> SMDEAVGDLKQALPCVAESPTVHVEVHQRGSSTAKKEDINLSVRKLLNRHNIVFGDYTWTEFDEPFLTRNVQSVSIIDTELKVKDSQPIDLSACTVALHIFQLNEDGPSSENLEEETENIIAANHWVLPAAEFHGLWDSLVYDVEVKSHLLDYVMTTLLFSDKNVNSNLITWNRVVLLHGPPGTGKTSLCKALAQKLTIRLSSRYRYGQLIEINSH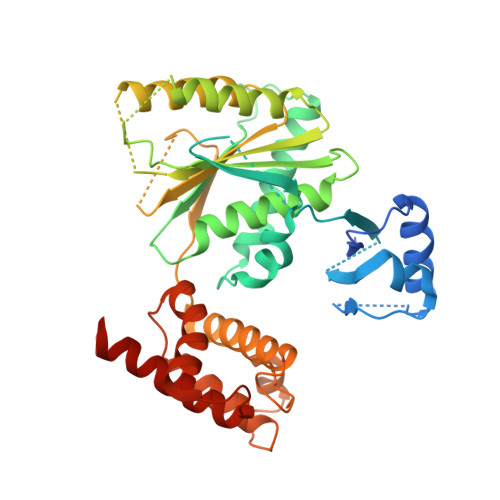SLFSKWFSESGKLVTKMFQKIQDLIDDKDALVFVLIDEVESLTAARNACRAGTEPSDAIRVVNAVLTQIDQIKRHSNVVILTTSNITEKIDVAFVDRADIKQYIGPPSAAAIFKIYLSCLEELMKCQIIYPRQQLLTLRELEMIGFIENNVSKLSLLLNDISRKSEGLSGRVLRKLPFLAHALYVQAPTVTIEGFLQALSLAVDKQFEERKKLAAYI>MMLSLRPYEFWFVTGSQHLYGEEALKQVEEHSRIMVNEWNRDSVFPFPFVFKSVVTTPEEIRRVCLEANASEQCAGVVTWMHTFSPAKMWIGGLLELRKPLLHLHTQFNRDIPWDSIDMDFMNLNQSAHGDREFGFMVTRLGMPRKVIVGHWQDAEVARRVRGWAMTAVAAAVSRGLKVARFGDNMRQVAVTEGDKVEAEARFGWSVNGYGVGDLAERVRAVSEAEIDRLIDEYQSLYEFAPGCEKGGPLHDGVREQARIELGLRSFLEEGGFEAFTTTF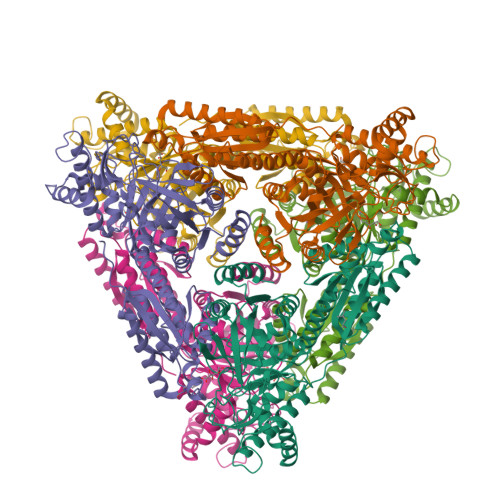EDLHGMKQLPGLAVQRLMAEGYGFGGEGDWKTAALVRLMKVMADGKGTSFMEDYTYHFEPGNEMILGAHMLEVCPTIAATRPRIEVHPLSIGGKEDPARLVFDGGEGAAVNASLIDLGHRFRLIVNEVDAVKPEHDMPKLPVARILWKPRPSLRDSAEAWILAGGAHHTCFSFAVTTEQLQDFAEMAGIECVVINEHTSVSSFKNELKWNEVFWRGR[6x]>[4x]EIPLKYGATNEGKRQDPAMQKFRDNRLGAFIHWGLYAIPGGEWNGKVYGGAAEWLKSWAKVPADEWLKLMDQWNPTKFDAKKWAKMAKEMGTKYVKITTKHHEGFCLWPSKYTKYTVANTPYKRDILGELVKAYNDEGIDVHFYFSVMDWSNPDYRYDI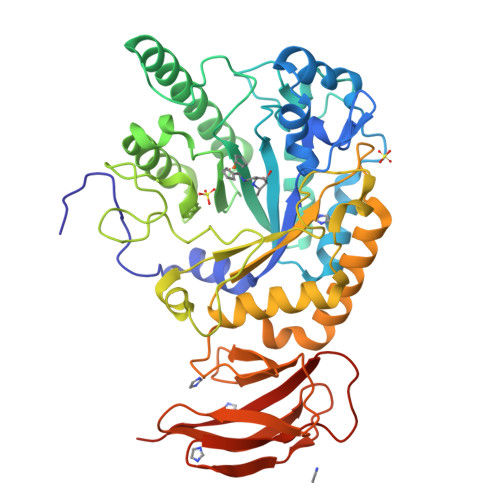KSKEDSIAFSRFLEFTDNQLKELATRYPTVKDFWFDGTWDASVKKNGWWTAHAEQMLKELVPGVAINSRLRADDKGKRHFDSNGRLMGDYESGYERRLPDPVKDLKVTQWDWEACMTIPENQWGYHKDWSLSYVKTPIEVIDRIVHAVSMGGNMVVNFGPQADGDFRPEEKAMATAIGKWMNRYGKAVYACDYAGFEKQDWGYYTRGKNDEVYMVVFNQPYSERLIVKTPKGITVEKATLLTTGEDITVVETTRNEYNVSVPKKNPGEPYVIQLKVRAAKGTKSIYRDALT> VDLVRTKVYNLLKEMILNHELKLGEKLNVRELSEKLGISFTPVRDALLQLATEGLVKVVPRVGFFVTDVDEKFIRETIETRIMMEVFCLENYFDKIAGSEELLEIKGEIDDVAASAAREIFDDSDERLHKLFIRASGNELIISLYEKIWDRIDLVRHLNERYVVSNREHKELIE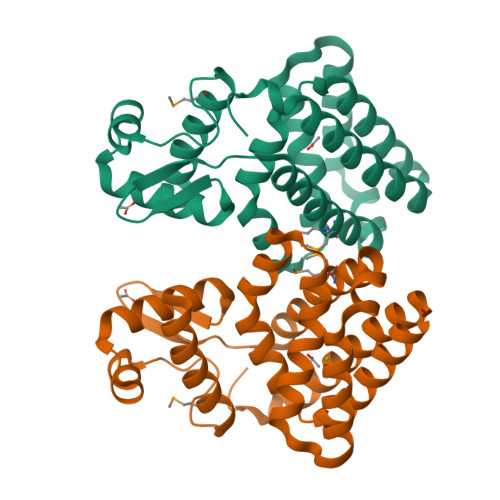RIISGDKEGAIEKLKEHLKNVEAETIKNLYTYERS> GSAMGSASTSGNPFQANVEMKTFMERFNLTHHHQSGIYVDLGQDKEVDGTLY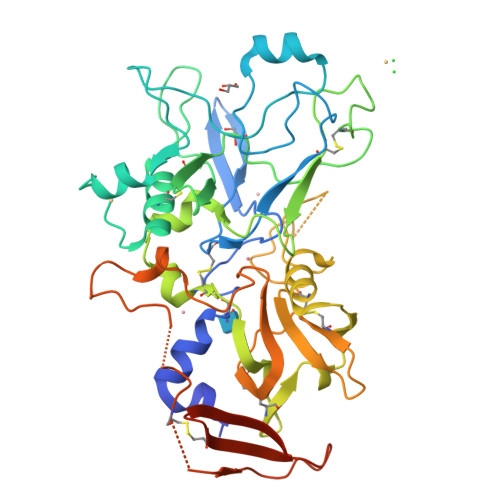REPAGLCPIWGKHIELQQPDRPPYRNNFLEDVPTEKEYKQSGNPLPGGFNLNFVTPSGQRISPFPMELLEKNSNIKASTDLGRCAEFAFKTVAMDKNNKATKYRYPFVYDSKKRLCHILYVSMQLMEGKKYCSVKGEPPDLTWYCFKPRKSVTENHHLIYGSAYVGENPDAFISKCPNQALRGYRFGVWKKGRCLDYTELTDTVIERVESKAQCWVKTFENDGVASDQPGSGSGSGDQPHSGGVGRNYGFYYVDTTGEGKCALSDQVPDCLVSDSAAVSYTAAGSLSEETPNFIIPSNPSVTPPTPETALQCTADKFPDSFGACDVQACKRQKTSCVGGQIQSTSVDCTADEQNECGSNTAAALVPR>SRLVVVSNRIAPPDEHAASAGGLAVGILGALKAAGGLWFGWSGETGNEDQPLKKVKKGNITWASFNLSEQDLDEYYNQFSNAVLWPAFHYRLDLVQFQRPAWDGYLRVNALLADKLLPLLQDDDIIWIHDYHLLPFAHELRKRGVNNRIGFFLHIPFPTPEIFNALPTYDTLLEQLCDYDLLGFQTENDRLAFLDCLSNLTRVTTRSAKSHTAWGKAFRTEVYPIGIEPKEIAKQAAGPLPPKLAQLKAELKNVQNIFSVERLDYSKGLPERFLAYEALLEKYPQHHGKIRYTQIAPTSRGDVQAYQDIRHQLENEAGRINGKYGQLGWTPLYYLNQH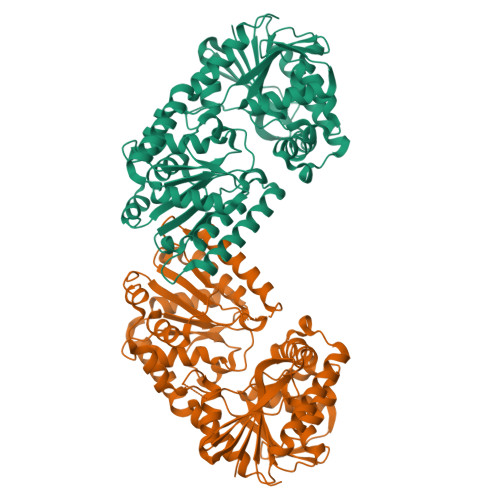FDRKLLMKIFRYSDVGLVTPLRDGMNLVAKEYVAAQDPANPGVLVLSQFAGAANELTSALIVNPYDRDEVAAALDRALTMSLAERISRHAEMLDVIVKNDINHWQECFISDLKQIVP[4x]>[6x]MTLSIIVAHDKQRVIGYQNQLPWHLPNDLKHIKQLTTGN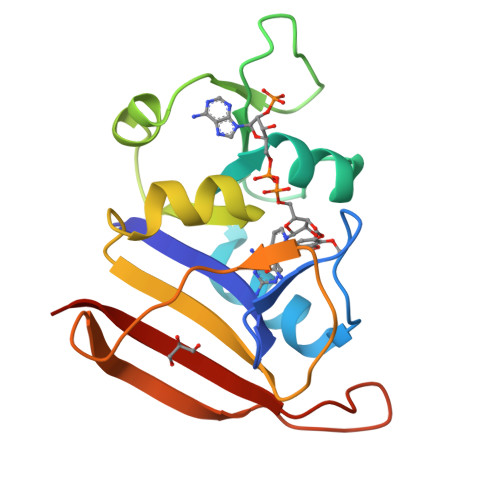TLVMARKTFESIGKPLPNRRNVVLTNQASFHHEGVDVINSLDEIKELSGHVFIFGGQTLYEAMIDQVDDMYITVIDGKFQGDTFFPPYTFEDWEVESSVEGQLDEKNTIPHTFLHLVRRKGK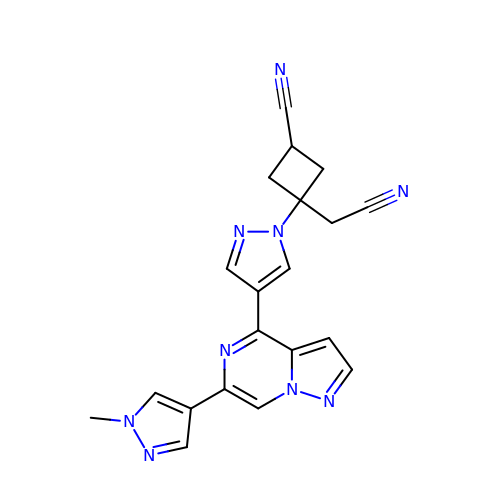trans-3-(cyanomethyl)-3-{4-[6-(1-methyl-1H-pyrazol-4-yl)pyrazolo[1,5-a]pyrazin-4-yl]-1H-pyrazol-1-yl}cyclobutane-1-carbonitrile | C20 H17 N9 | XPLZTJWZDBFWDE-OYOVHJISSA-N>GMSVKVSVDDIDGITEVLNVYMNAAESGTGEEMSAAFHKDATIFGYVGDKLAFNGPIKDLYDWHNSNGPAKNVQSRITNIDIVGTVAHARVEAENWTNFKFSDLFLLLKLDGKWTIVNKVFHL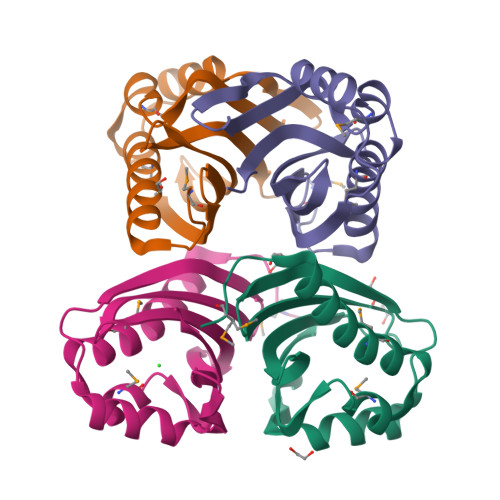HA[6x]>SNAMIRQARPEDRFDIAKLVYMVWDDMELELVKHLPKDMVLDAIEKSCVDATYRTFYQHILVYEVENKVAGCIISYSGENELKYEKAWELLDLPEEIKQYGTPLPVKEAKDDEYYIETIATFAAYRGRGIATKLLTSLLESNTHVKWSLNCDINNEAALKLYKKVGFISDGQIELYKHMYHHLIVK[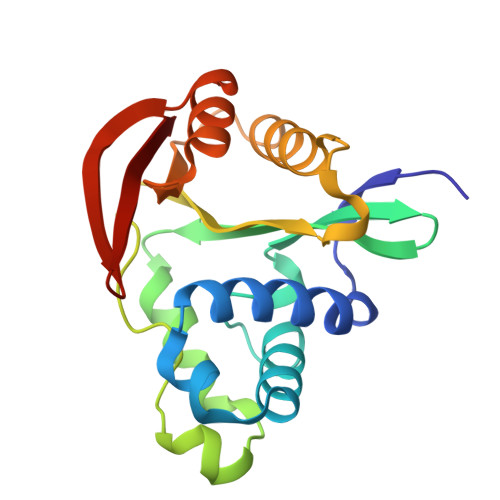4x]Bromodomains (BRDs) are protein interaction modules that specifically recognize ε-N-lysine acetylation motifs, a key event in the reading process of epigenetic marks. The 61 BRDs in the human genome cluster into eight families based on structure/sequence similarity. Despite large sequence variations, all BRD modules share a conserved fold that comprises a left-handed bundle of four α helices (αZ, αA, αB, αC), linked by loop regions of variable length (ZA and BC loops), which line the Kac binding site and determine binding specificity. The four helices form a deep cavity that is extended by the two loop regions (ZA and BC loops), creating a largely hydrophobic Kac binding pocket.

BRDs are evolutionarily conserved and present in diverse nuclear proteins comprising HATs (GCN5, PCAF), ATP-dependent chromatin-remodeling complexes (BAZ1B), helicases (SMARCA), methyltransferases (MLL, ASH1L), transcriptional coactivators (TRIM/TIF1, TAFs) transcriptional mediators (TAF1), nuclear-scaffolding proteins (PB1), and the BET family (Muller et al., 2011).

>SMEDPDQLYTTLKNLLAQIKSHPSAWPFMEPVKKSEAPDYYEVIRFPIDLKTMTERLRSRYYVTRKLFVADLQRVIANCREYNPPDSEYCRCASALEKFFYFKLKEGGLIDK[2x]> MTSRFGKTYSRKGG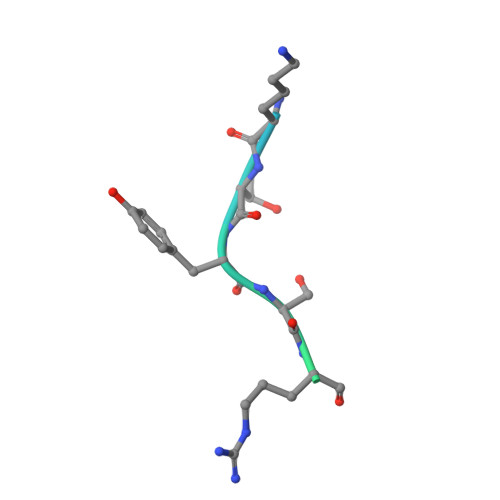NGSSKFDEVFSNKRTTLST>MADSNGTITVEELKKLLEQWNLVIGFLFLTWICLLQFAYANRNRFLYIIKLIFLWLLWPVTLACFVLAAVYRINWITGGIAIAMACLVGLMWLSYFIASFRLFARTRSMWSFNPETNILLNVPLHGTILTRPLLESELVIGAVILRGHLRIAGHHLGRCDIKDL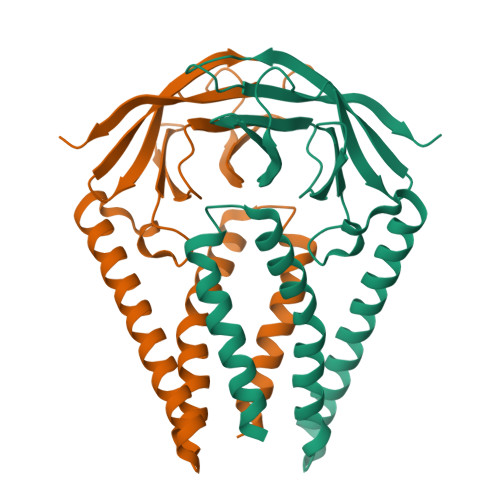PKEITVATSRTLSYYKLGASQRVAGDSGFAAYSRYRIGNYKLNTDHSSSSDNIALLVQSNSLEVLFQ[2x]>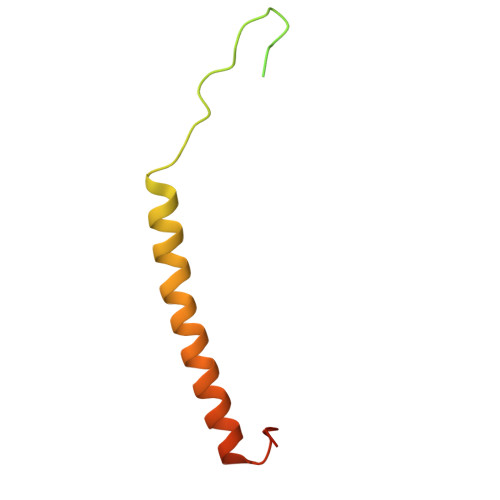 MASGAARWLVLAPVRSGALRSGPSLRKDGDVSAAWSGSGRSLVPSRSVIVTRSGAILPKPVKMSFGLLRVFSIVIPFLYVGTLISKNFAALLEEHDIFVPEDDDDDD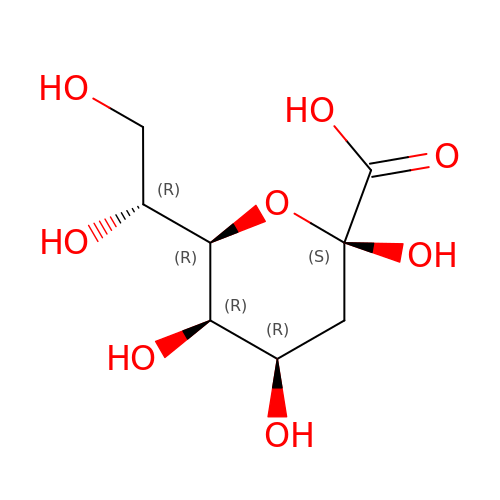3-deoxy-beta-D-manno-oct-2-ulopyranosonic acid | C8 H14 O8 | NNLZBVFSCVTSLA-FBXMPTEYSA-N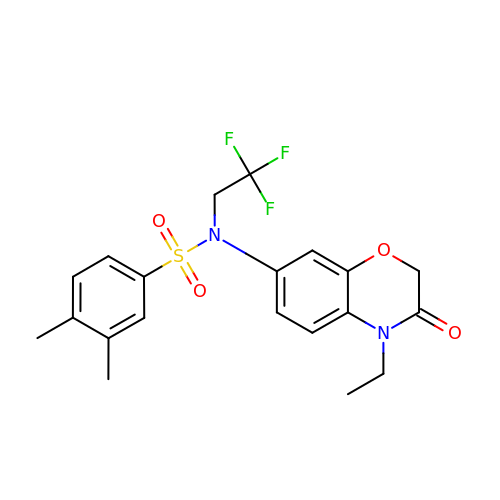N-(4-ethyl-3-oxo-3,4-dihydro-2H-1,4-benzoxazin-7-yl)-3,4-dimethyl-N-(2,2,2-trifluoroethyl)benzene-1-sulfonamide | C20 H21 F3 N2 O4 S | LODXRGHOWOQXTP-UHFFFAOYSA-N> MAHHHHHHSSGLEVLFQGPYDQVDQLGVNTLRTLSIDAIQRANSGHPGLPMGAAPMAYVLWTRHLKINPKTHMNWVNRDRFVLSAGHGSALLYSLAHLAGYDVSMDDLKNFREWKSNTPGHPEYGCTDGVEATTGPLGQGISMAVGMAMAEAHLGKKFNREGYPVMDHYTYALIGDGDLMEGVASEAASLAGHLKLGKLIALYDSNGISLDGKTSASFTENVGARFEAYGWQYILVEDGFNLEEIDKAIVQAKAESDKPTIIEIKTTIGYGSENQGTHKVHGSPLGEEGVAHAKEVYNWNYPPFTVPEEVSQRFKECLQDKGVKAENKWNEMFEAYKKEYSDLAQKFSDGFSNKVPNTLGDILPQYGEDDSIATRAASQKAINALAKEVSSLWGGAADLASSNKTVIAGEGDFQPESYEGRNIWFGVREFGMACAMNGIMLHGGTRIFGSTFFVFSDYLKAAIRLSAIQKLPVIYVLTHD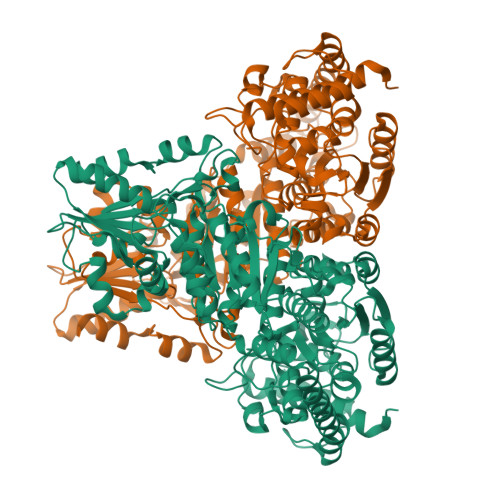SVAVGKDGPTHEPIEQLASLRTIPNVQVFRPADGNETSAAWKVALETLDKPTILVLSRQNLDTLPISKEKVFDGVEKGGYVVQGAENEADGILIATGSEVGLALKAKEELQKKGKDVIVVSLPSWERFEAQSEEYKNTVIPPELKKRMTIEAGTTYGWAKYAGDHGVMIGIDEFGMSAPSDIVLRELGMSVENIVDKYLEK>MSKAGASLATCYGPVSADVMAKAENIRLLILDVDGVLSDGLIYMGNNGEELKAFNVRDGYGIRCALTSDIEVAIITGRKAKLVEDRCATLGITHLYQGQSNKLIAFSDLLEKLAIAPENVAYVGDDLIDWPVMEKVGLSVAVADAHPLLIPRADYVTRIAGGRGAV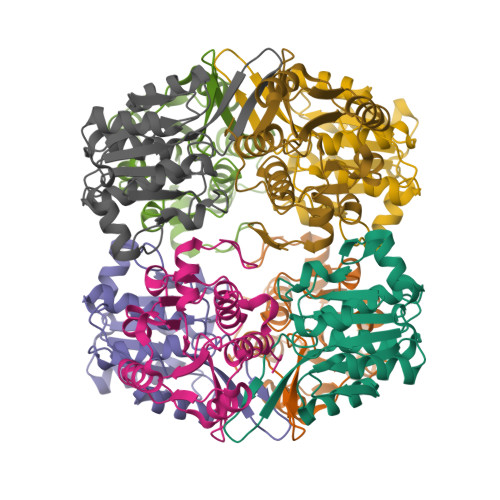REVCDLLLLAQGKLDEAKGQSI[16x]>ADLPALPGGPAGGTGELAKYGLPGVAQLRSRESYVLSYDPRTRGALWVLEQLRPERLRGDGDRSACDFREDDSVHAYHRATNADYRGSGFDRGALAAAANHRWSQRAMDDTFYLSNVAPQVPHLNQNAWNNLERYSRSLTRTYQNVYVCTGPLFLPRTEADGKSYVKYQVIGKNHVAVPTHFFKVLILEAAGGQIELRSYVMPNAPVDETIP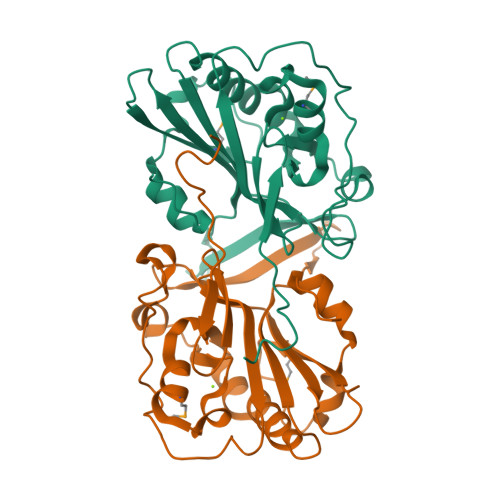LERFLVPIESIERASGLLFVPNILARAGNLKAITAGS[4x]>[6x]MILIADSGSTKTDWCVVLNGAVIKRLGTKGINPFFQSEEEIQQKLTASLLPQLPEGKFNAVYFYGAGCTPEKAPVLRRA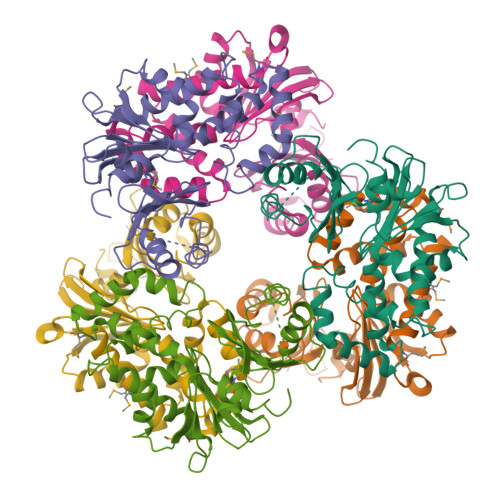IADSLPVIGNIKANSDMLAAAHGLCGQKAGIACILGTGSNSCFYNGKEIVSNISPLGFILGDEGSGAVLGKLLVGDILKNQLPATLKEEFLKQFDLTPPEIIDRVYRQPFPNRFLASLSPFIAQHLEEPAIRQLVMNSFIAFFRRNVMQYDYKQYPVHFIGSIAYCYKEILQDAARQTGIQIGKILQSPMEGLIQYHSQLSFHPLEHHHHHH>LPDLKIEKLEEGVFVHTSFEEVNGWGVVTKHGLVVLVNTDAYLIDTPFTATDTEKLVNWFVERGYEIKGTISSHFHSDSTGGIEWLNSQSIPTYASELTNELLKKSGKVQAKYSFSEVSYWLVKNKIEVFYPGPGHTQDNLVVWLPESKILFGGCFIKPHGLGNLGDANLEAWPKSAKILMSKYGKAKLVVSSHSEKGDASLMKRTWEQALKGLKESK[2x]

IMP-13, a member of subgroup 2, sharing 92.3% amino acid sequence similarity with IMP-2 and 82.5% with IMP-1 (Fig. SI2), was first identified in the Gram-negative pathogen Pseudomonas aeruginosa from clinical samples in Italy and is a common cause of carbapenem resistance, often involved in large outbreaks. Imipenemases represent one of the major groups of class B1 metallo-β-lactamases found in Gram-negative pathogens, and these enzymes can hydrolyze all bicyclic β-lactam antibiotics. The overall protein architecture of the IMP-13 apo structure is consistent with that of the previously published metallo-β-lactamase fold, consisting of a global αβ/βα topology with a shallow active-site cleft at the border of the two β-sheets. The structural information and dynamics presented here reveal important information about the mechanism of antibiotic binding, as well as a significant role for the active-site-covering loop (L1), indicating that the plasticity of the active-site region is important for the broad substrate recognition spectrum of these enzymes.

In the apo-state crystal structures, two positions for the L1 loop, open and closed, were observed. The L1 loop adopts very different conformations in the two apo structures (apoclosed and apoopen). In the apoclosed structure, the loop is folded over the active site, while in the apoopen structure, L1 is extended away from the protein, leaving the active site accessible. We define the open conformation to be the loop pointing away from the protein toward the solvent and the closed conformation to be the loop positioned over the active site and pointing toward its rim. The distance between C-α atoms of Trp28 for the open and closed conformations is 8.8 Å. A comparison of the carbapenem-bound complex structures with apoclosed elicits very few distinct differences, with the L1 loop seen to be packed over the antibiotic binding pocket. The distinct conformations observed in the two apo crystal structures and the NMR relaxation data indicate that the L1 loop is likely flexible in solution. The lower root mean squared fluctuations (RMSFs) for heavy atoms of L1 residues in the simulated doripenem-, ertapenem-, and meropenem-bound complex structures than for those of the apoclosed structure indicate that L1 is more rigid in the closed conformation when these ligands are bound, while in the apo protein, L1 can move with a higher degree of freedom.> SQAEVLHLCRSLEVGTVMTLFYSKKSQRPERKTFQVKLETRQITWSRGADKIEGSIDIREIKEIRPGKTSRDFDRYQEDPAFRPDQSHCFVILYGMEFRLKTLSLQATSEDEVNMWIKGLTWLMEDTLQAATPLQIERWLRKQFYSVDRNREDRISAKDLKNMLSQVNYRVPNMRFLRERLTDFEQRSGDITYGQFAQLYRSLMYSAQKTMDLPFLETNTLRTGERPELCQVSLSEFQQFLLEYQGELWAVDRLQVQEFMLSFLRDPLREIEEPYFFLDELVTFLFSKENSVWNSQLDAVCPETMNNPLSHYWISSSHNTYLTGDQFSSESSLEAYARCLRMGCRCIELDCWDGPDGMPVIYHGHTLTTKIKFSDVLHTIKEHAFVASEYPVILSIEDHCSIAQQRNMAQHFRKVLGDTLLTKPVDIAADGLPSPNQLKRKILIKHKKLAEGSAYEEVPTSVMYSENDISNSIKNGILYLEDPVNHEWYPHYFVLTSSKIYYSEETSSDQGNEDEEEPKEASGSTELHSSEKWFHGKLGAGRDGRHIAERLLTEYCIETGAPDGSFLVRESETFVGDYTLSFWRNGKVQHCRIHSRQDAGTPKFFLTDNLVFDSLYDLITHYQQVPLRCNEFEMRLSEPVPQTNAHESKEWYHASLTRAQAEHMLMRVPRDGAFLVRKRNEPNSYAISFRAEGKIKHCRVQQEGQTVMLGNSEFDSLVDLISYYEKHPLYRKMKLRYPINEEALEKIGSGSTFKCAVKALFDYKAQREDELTFTKSAIIQNVEKQDGGWWRGDYGGKKQLWFPSNYVEEMINPAILEPEREHLDENSPLGDLLRGVLDVPACQIAIRPEGKNNRLFVFSISMPSVAQWSLDVAADSQEELQDWVKKIREVAQTADARLTEGKMMERRKKIA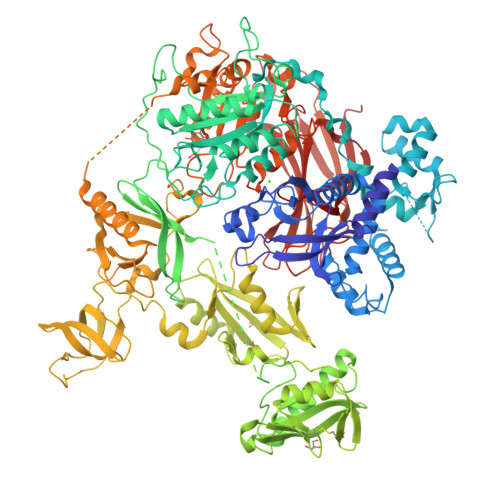LELSELVVYCRPVPFDEEKIGTERACYRDMSSFPETKAEKYVNKAKGKKFLQYNRLQLSRIYPKGQRLDSSNYDPLPMWICGSQLVALNFQTPDKPMQMNQALFMAGGHCGYVLQPSTMRDEAFDPFDKSSLRGLEPCVICIEVLGARHLPKNGRGIVCPFVEIEVAGAEYDSTKQKTEFVVDNGLNPVWPAKPFHFQISNPEFAFLRFVVYEEDMFSDQNFLAQATFPVKGLKTGYRAVPLKNNYSEDLELASLLIKIDIFPAK> MAHSRASTKVVVVGGGGTIGSSTALHLIRRGYTPSNITVLDVYKTPSLQSAGHDLNKIMSIRLRNGPDLQLSLESLDMWQNDELFKPFFHQVGMLDCSSSKEGIENLRRKYQTLLDAGIGLEKTNVWLESEDEILAKVPNFTREQVKGWKGLFCTDGGWLAAAKAINAIGIFLQDKGVKFGFGDAGTFQQPLFAADGKTCIGLETTDGTKYFADKVVLAAGAWSPTLVDLEDQCVSKA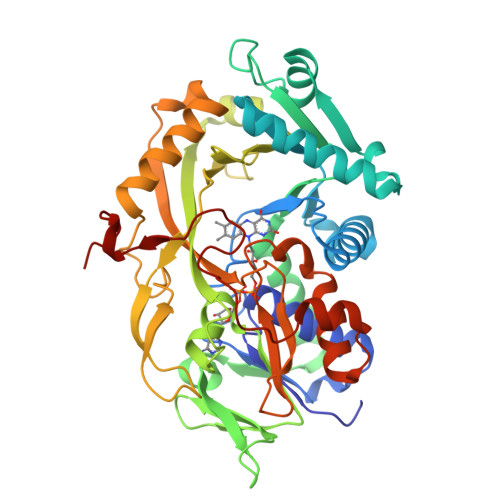WVFAHIQLTPKEADAYKNVPVVYDGEYGFFFEPNEYGVIKVCDEFPGYSRFKLHQPYGAASPKMISVPRSHAKHPTDTYPDASEVTIRKAIARFLPEFKDKELFNRTMCWCTDTADANLLICEHPKWKNFILATGDSGHSFKLLPNIGKYVVELLEGSLSQEMAGAWRWRPGGDALRSRRGAPAKDLAEMPGWKHDAHL> MKKMVFCKMCRPLLVFCATSCWRRSARLPLPFFFSPLNLQVAPFTSWNLQARYFSTTAGGGREGTNSSEDDYVFDPTLSVQKDAAIHVAKKSLDAIVRDLLPENAPDAATQKVRAYLQQHPMDTLITQPTVHITHVEDPESGRETKMSLSPCDLSEALEQAQEREMNLVQMGTRGDVAYCRIRREIPRILGLVGPELEALREEEKQEGSSHRGGSDQAGGKIRELVDHSFRDVVDAHFVGWKSKKIVEDIKKRHPV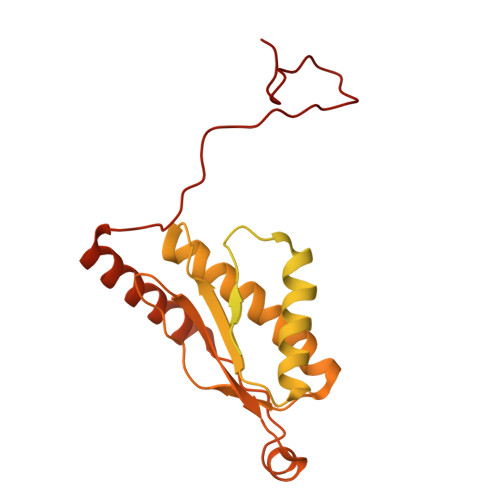KITIKEFQSPEAAIGKIREMCQAMQRYAEEKLIYHHFTSIVANDREVSVSFVPSLPSEKGNSWKHIKYPGEKEWAHANKRMEEACRKSGRYGTYVKNNMLKPRSLGQTFFRVDKYGRKID In the PT-based defense system Ssp, SspABCD confers a single-stranded PT modification of host DNA in the 5′-CPSCA-3′ motif and SspE impedes phage propagation. Notably, SspABCD coupled with SspE confers resistance to a wide array of phages through unusual mechanisms: (1) SspE is a dual-function protein that exerts both N-terminal NTPase and C-terminal DNA nicking nuclease activities to defend against phage infection, and (2) NTPase activity, including GTPase, CTPase, and UTPase activity, is stimulated exclusively by 5′-CPSCA-3′-containing DNA in vitro. Here, structural and biochemical analyses reveal that SspE is preferentially recruited to PT sites mediated by the joint action of its N-terminal domain (NTD) hydrophobic cavity and C-terminal domain (CTD) DNA binding region. PT recognition enlarges the GTP-binding pocket, thereby increasing GTP hydrolysis activity, which subsequently triggers a conformational switch of SspE from a closed to an open state.

The full-length SspE structure revealed a smaller NTD (residues 1 to 324) and a larger CTD (residues 332 to 771), which were connected by a short linker of only seven residues T325TGQPLT331. The NTD of SspE exhibited a DUF262-fold with the strongly conserved D96GQQR100 signature motif, which was essential for GTP hydrolysis and was positioned at the junction of the α3 helix and the β4 strand. The CTD of SspE contains a DUF1524 domain that belongs to the His-Asn-His (HNH, the last histidine of which can be replaced by an asparagine, as observed in SspE) nuclease superfamily and indeed exerts DNA nickase activity in vitro. In contrast to the typical HNH motif in Cas9, GVE2, ScoMcrA16, ColE7, or BrxU18 that consists of two antiparallel β-sheets and an α-helix, the HNH motif in the CTD of SspE from S. yokosukanensis DSM 40224 was composed of two antiparallel β-sheets and a loop, suggesting comparatively higher flexibility. However, the active sites of the HNH motif in SspE still adopt a characteristic ββα-metal topology, in which the first histidine typically acts as the general base in the DNA cleavage reaction, asparagine is involved in structural stabilization and the third residue, which can be either histidine or asparagine, is responsible for metal binding. Indeed, single-point substitution of N676 in the HNH motif by an alanine or the elimination of divalent metal cations, i.e., Mg2+, markedly impaired the DNA nicking activity of SspE in vitro. One unique hydrophobic patch that was also lined with positively charged residues, e.g., R32, was located on the surface of the N-terminal region of the SspE structure. SspE displayed an extended dumbbell-like shape, with a short loop linking its two globular NTD and CTD domains. The NTD and CTD packed loosely against each other, with few contacts between them.

>[4x]METKEIFDAAPLSVSQFLSETGQGLYIPPYQRAYSWELPKIRRLLSDVAHGLDQLAEFEDSICFLGTVIALRDINYTTVEPKYRSQVPSKVMTIIDGQQRMTTLLLLTTVLHEEIRVRAEKLTRDDEPSVWCYNQALDVTGRLSNCFEEDMRYGEHRYYPRLIRSYYDVWSRNKGEARYRSPIGYYLESYGAYARDPDAVKPYRHVPIDPDKTDGVDLEAYRHLDRMRDQMRSMLRKAVGAGVKREDDIQLPTGTDIGQSQNLQFALFNSEFPPSVVEQLEDDAKMTPLTRLIVFANYLLHRVTVAVVTAKREDYGFDMFEALNTTGQPLTAIETFKPRAIKEEGLDEWQESESKLHFDVVEAYLDREGSSSADKRQTVTSSVLLPFAMFQDGTKLTKRLNDQRRYLRTVFDKDPDIVARRKVLAGLAQVARFYEGPWGSPTKVPSCDDATLRTQAGIALAALREGGHDIVVGLLTRYFAAHRLSSPETVESSARQFLLAARSCAAFYALWRGSFGSTAGIDGVYRSLMTHVVEEGMPRFARFERDLTEVPPVEALQSYLKEQLRSEGIYDKQQWVARAAMTPVYQHSKPLTRLLLLAASQNSTPDSATPGLVVRGKSGLLETLELERWNDEAFATIEHVAPQAPSSNGSWNADLYEDPELINRIGNLTLLPAVENASASNRAWHLKRLMFRALSAATVEEAEKTLADAEAQGLRLGSGAGEIVRQARYLPLVAALAQREEEWTAEFVEARSQRLCSLAWDALTPWLGFEP> MPTGSVTVRVPGKVNLYLAVGDRREDGYHELTTVFHAVS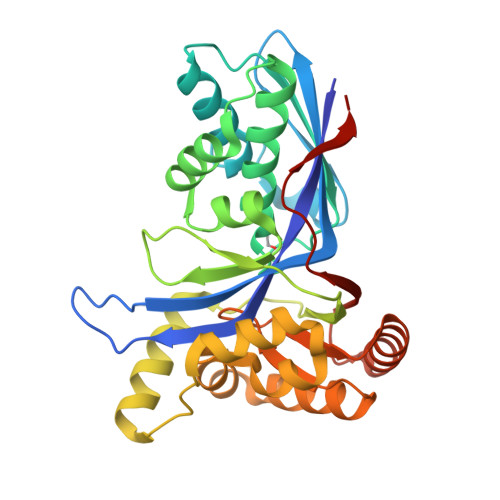LVDEVTVRNADVLSLELVGEGADQLPTDERNLAWQAAELMAEHVGRAPDVSIMIDKSIPVAGGMAGGSADAAAVLVAMNSLWELNVPRRDLRMLAARLGSDVPFALHGGTALGTGRGEELATVLSRNTFHWVLAFADSGLLTSAVYNELDRLREVGDPPRLGEPGPVLAALAAGDPDQLAPLLGNEMQAAAVSLDPALARALRAGVEAGALAGIVSGSGPTCAFLCTSASSAIDVGAQLSGAGVCRTVRVATGPVPGARVVSAPTEV>[2x]GGIKMDTQFYDSFTFDNVKYSLYDNVYLFKSGESEP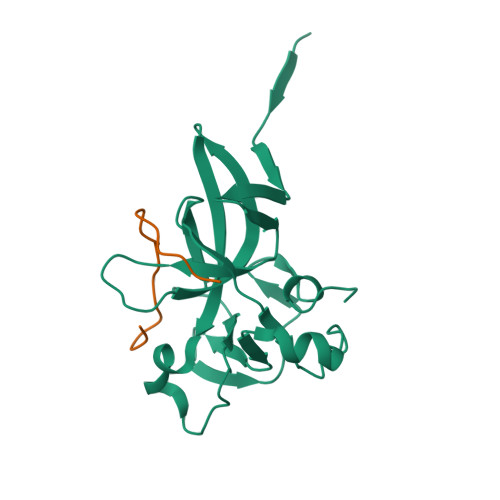YIGKIIKIWQQNQAKKVKILWFFLPDEIRKHLSGPVMEKEIFLACGEGVGLADINPLEAIGGKCTVLCISKDERNRQPSPRELAMADYIFYRFFDVNSCTLSEQLPEKIAGVEGNLLLNSKVE;>[2x]PPKRRAISAIRKFPRDCG> ATTCTFSGSNGASSASKSKTSCSTIVLSNVAVPSGTTLDLTKLNDGTHVIFSGETTFGYKEWSGPLISVSGSDLTITGASGHSINGDGSRWWDGEGGNGGKTKPKFFAAHSLTNSVISGLKIVNSPVQVFSVAGSDYLTLKDITIDNSDGDDNGGHNTDAFDIGTST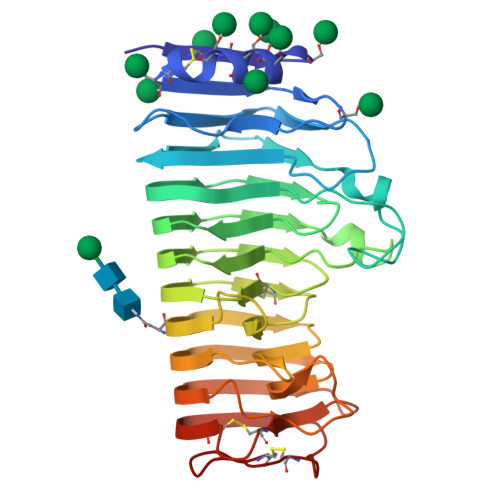YVTISGATVYNQDDCVAVNSGENIYFSGGYCSGGHGLSIGSVGGRSDNTVKNVTFVDSTIINSDNGVRIKTNIDTTGSVSDVTYKDITLTSIAKYGIVVQQNYGDTSSTPTTGVPITDFVLDNVHGSVVSSGTNILISCGSGSCSDWTWTDVSVSGGKTSSKCTNVPSGASC>[8x]MGHHHHHHVSSTNGFSATRSTVIQLLNNISTKREVEQYLKYFTSVSQQQFAVIKVGGAIISDNLHELASCLAFLYHVGLYPIVLHGTGPQVNGRLEAQGIEPDYIDGIRITDEHTMAVVRKCFLEQNLKLVTALEQLGVRARPITSGVFTADYLDKDKYKLVGNIKSVTKEPIEASIKAGALPILTSLAETASGQMLNVNADVAAGELA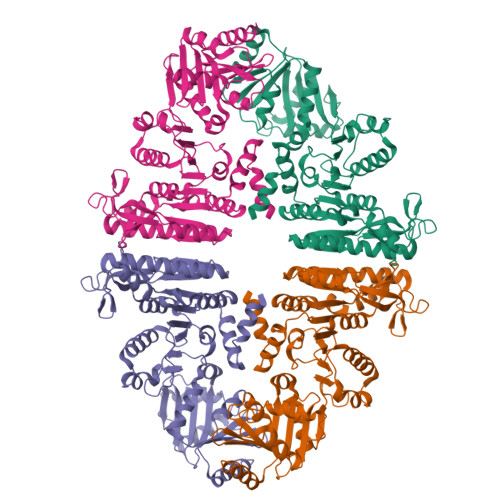RVFEPLKIVYLNEKGGIINGSTGEKISMINLDEEYDDLMKQSWVKYGTKLKIREIKELLDYLPRSSSVAIINVQDLQKELFTDSGAGTMIRRGYKLVKRSSIGEFPSADALRKALQRDAGISSGKESVASYLRYLENSDFVSYADEPLEAVAIVKKDTNVPTLDKFVCSDAAWLNNVTDNVFNVLRRDFPALQWVVSENDANIAWHFDKSQGSYLKGGKVLFWYGIDDINTISELVENFVKSCDTASTLNSSASS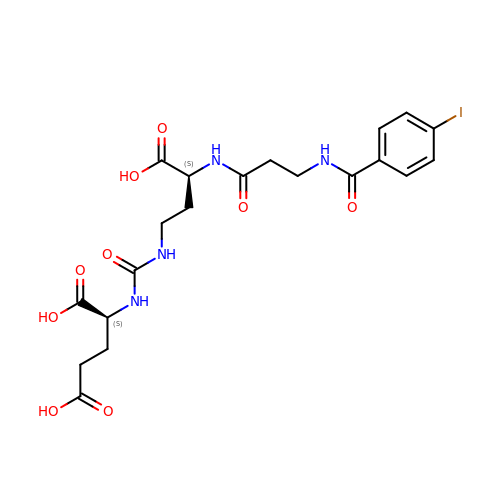(2~{S})-2-[[(3~{S})-3-[3-[(4-iodophenyl)carbonylamino]propanoylamino]-4-oxidanyl-4-oxidanylidene-butyl]carbamoylamino]pentanedioic acid | C20 H25 I N4 O9 | GMICYHSMDRPTBB-KBPBESRZSA-N> MSLAVLLNKEDKDISDFSKTTAGKSAKKNSRERVADVAPTRVLDKKQAYLSQLNSEFNRIKRRDSIEQLYQDWKFINLQEFELISEWNQQSKDWQFDNTNDSQDLHFKKLYRDMSMINKEWAEYQSFKNANLSDIINEKDADEDEEDDEDELEDGEEDMEEDEASTGRHTNGKSMRGNGIQKSRKKDAAAAAAIGKAIKDDQTHADTVVTVNGDENEDGNNGEDEDNDNDNENNNDNDNDNENENDNDSDNDDEEENGEEDEEEEEIEDLDEEDFAAFEEQDDNDDEDFNPDVEKRRKRSSSSSSSTKLSMNSLSLITSKKINKNITINSDRPKIVRELIKMCNKNKHQKIKKRRFTNCIVTDYNPIDSKLNIKITLKQYHVKRLKKLINDAKREREREEALKNNVGLDGNDLDNDEDGSESHKRRKLNNNTANGADDANKRKFNTRHGLPTYGMKMNAKEARAIQRHYDNTYTTIWKDMARKDSTKMSRLVQQIQSIRSTNFRKTSSLCAREAKKWQSKNFKQIKDFQTRARRGIREMSNFWKKNEREERDLKKKIEKEAMEQAKKEEEEKESKRQAKKLNFLLTQTELYSHFIGRKIKTNELEGNNVSSNDSESQKNIDISALAPNKNDFHAIDFDNENDEQLRLRAAENASNALAETRAKAKQFDDHANAHEEEEEEDELNFQNPTSLGEITIEQPKILACTLKEYQLKGLNWLANLYDQGINGILADEMGLGKTVQSISVLAHLAENHNIWGPFLVVTPASTLHNWVNEISKFLPQFKILPYWGNANDRKVLRKFWDRKNLRYNKNAPFHVMVTSYQMVVTDANYLQKMKWQYMILDEAQAIKSSQSSRWKNLLSFHCRNRLLLTGTPIQNSMQELWALLHFIMPSLFDSHDEFNEWFSKDIESHAEANTKLNQQQLRRLHMILKPFMLRRVKKNVQSELGDKIEIDVLCDLTQRQAKLYQVLKSQISTNYDAIENAATNDSTSNSASNSGSDQNLINAVMQFRKVCNHPDLFERADVDSPFSFTTFGKTTSMLTASVANNNSSVISNSNMNLSSMSSNNISNGKFTDLIYSSRNPIKYSLPRLIYEDLILPNYNNDVDIANKLKNVKFNIFNPSTNYELCLFLSKLTGEPSLNEFFRVSTTPLLKRVIERTNGPKNTDSLSFKTITQELLEVTRNAPSEGVMASLLNVEKHAYEREYLNCIQRGYHPNVSAPPVTIEVLGSSHVTNSINNELFDPLISQALSDIPAITQYNMHVKKGIPVEDFPKTGLFPEPLNKNFSSNISMPSMDRFITESAKLRKLDELLVKLKSEGHRVLIYFQMTKMMDLMEEYLTYRQYNHIRLDGSSKLEDRRDLVHDWQTNPEIFVFLLSTRAGGLGINLTAADTVIFYDSDWNPTIDSQAMDRAHRLGQTRQVTVYRLLVRGTIEERMRDRAKQKEQVQQVVMEGKTQEKNIKTIEVGENDSEVTREGSKSISQDGIKEAASALA;> MSSRDASLTPLKAVVIDDPPLRQTPEPFDEQSAYNPQSPIAIDFGSSKLRAGFVNHATPTHIFPNALTKFRDRKLNKNFTFVGNDTLLDQAVRSQSRSPFDGPFVTNWNLTEEILDYTFHHLGVVPDNGIPNPILLTERLATVQSQRTNWYQILFETYNVPGVTFGIDSLFSFYNYNPSGNKTGLVISCGHEDTNVIPVVDGAGILTDAKRINWGGHQAVDYLNDLMALKYPYFPTKMSYLQYETMYKDYCYVSRNYDEDIEKILTLENLDTNDVVVEAPFTEVLQPQKTEEELRIQAEKRKETGKRLQEQARLKRMEKLVQKQEEFEYFSKVRDQLIDEPKKKVLSVLQNAGFDDERDFKKYLHSLEQSLKKAQMVEAEDDSHLDEMNEDKTAQKFDLLDIADEDLNEDQIKEKRKQRFLKASQDARQKAKEEKERVAKEEEEKKLKEQQWRETDLNGWIKDKRLKLNKLIKRRKEKLKLRDEMKDRKSQVSQNRMKNLASLAEDNVKQGAKRNRHQATIDNDPNDTFGANDEDWLIYTDITQNPEAFEEALEYEYKDIVELERLLLEHDPNFTEEDTLEAQYDWRNSILHLFLRGPRPHDSENIHEQHQMHLNVERIRVPEVIFQPTMGGQDQAGICELSETILLKKFGSQPGKLSQTSIDMVNNVLITGGNAKVPGLKERIVKEFTGFLPTGTNITVNMSSDPSLDAWKGMAALARNEEQYRKTVISKKEYEEYGPEYIKEHKLGNTKYFED;> MSGSRGNSSNSSVSNNSNNNNNNDGGDERLLFLRSVGERNEIGFPSRFKSAHYKKPTRRHKSARQLISDENKRINALLTKANKAAESSTAARRLVPKATYFSVEAPPSIRPAKKYCDVTGLKGFYKSPTNNIRYHNAEIYQLIVKPMAPGVDQEYLKLRGANFVLK;>MVAISEVKENPGVNSSNSGAVTRTAAHTHIKGLGLDESGVAKRVEGGFVGQIEAREACGVIVDLIKAKKMSGRAILLAGGPSTGKTALALAISQELGPKVPFCPLVGSELYSVEVKKTETLMENFRRAIGLRIKETKEVYEGEVTELTPEDAENPLGGYGKTISHVIVGLKSAKGTKTLRLDPTIYESIQREKVSIGDVIYIEANTGAVKRVGRSDAYATEFDLETEEYVPLPKGEVHKKKEIVQDVTLHDLDVANARPQGGQDVISMMGQLLKPKKTEITEKLRQEVNKVVAKYIDQGVAELIPGVLFIDEVNMLDIEIFTYLNKALESNIAPVVVLASNRGMTTVRGTEDVISPHGVPPDLIDRLLIVRTLPYDKDEIRTIIERRATVERLQVESSALDLLATMGTETSLRYALQLLAPCGILAQTSNRKEIVVNDVNEAKLLFLDAKRSTKILETSANYL[3x];>MSIQTSDPNETSDLKSLSLIAAHSHITGLGLDENLQPRPTSEGMVGQLQARRAAGVILKMVQNGTIAGRAVLVAGPPSTGKTALAMGVSQSLGKDVPFTAIAGSEIFSLELSKTEALTQAFRKSIGIKIKEETELIEGEVVEIQIDRSITGGHKQGKLTIKTTDMETIYELGNKMIDGLTKEKVLAGDVISIDKASGKITKLGRSFARSRDYDAMGADTRFVQCPEGELQKRKTVVHTVSLHEIDVINSRTQGFLALFTGDTGEIRSEVRDQINTKVAEWKEEGKAEIVPGVLFIDEVHMLDIECFSFINRALEDEFAPIVMMATNRGVSKTRGTNYKSPHGLPLDLLDRSIIITTKSYNEQEIKTILSIRAQEEEVELSSDALDLLTKTGVETSLRYSSNLISVAQQIAMKRKNNTVEVEDVKRAYLLFLDSARSVKYVQENESQYIDDQGNVQISIAK[3x];> MDSEASDIEAELSDSVSAGGEEYIDDDDYTEDIDDQIVTAKSSRRTARRSVPKGVRTSKRIRDKELSVEVDEDYDEEEDVLSPSKKRHLHTRSMDKRQVAATASEKSDIGDSKGNDGEIEDGILEEEESLEKELNRGGGKEVEKSEESYYAQNDVGQKGEEEQDGESGGYEDNEPSISKESDELVSVVNGNGNEEDDEVEATKENTTDSTRSTTTRSKMLLDLLEDGGSKKKLTDEEIQLRRAENARKRKNLSEKRLEEEKQDTINKLLKKRAGKSRSHLPNDDEKNDGSSSFVKPRRPYNSEGMTRILRRYEEDLFCTF

However, amongst these remodelers, the INO80 chromatin remodeler appears largely sufficient to generate the well positioned +1 and −1 nucleosomes. S.c INO80 is a multi-subunit complex consisting of 15 subunits that are divided into three different modules. The catalytic module with the Ino80 (ATPase) RecA lobes and insert, Arp5, Ies6, Ies2, Rvb1 and Rvb2, constitutes the core unit of INO80 (C-module). INO80 slides nucleosomes with 40 bp of flanking DNA ~100-fold slower than nucleosomes with 80 bp of flanking DNA, displaying a switch like response to flanking DNA length.

INO80 complexes lacking the Arp8 module (ΔArp8) were purified from yeast strains lacking the Arp8 subunit, which results in the absence of the entire module. To test this possibility structurally, we determined the cryo-EM structure of ΔArp8 INO80 bound to S.c 0/40 nucleosomes in the presence of ADP/BeFx. The overall architecture of the C-module of ΔArp8 INO80 bound to 0/40 nucleosomes is again similar to that observed with WT INO80 bound to S.c 0/40 and 0/80. However, the density corresponding to the HSA around the Ino80 motor domain that was observed with the Arp8 module in WT INO80 is no longer detectable. This is likely because, without the Arp8 module, the HSA region is either poorly structured or highly dynamic. We interpret the absence of HSA density as indicative of an activated state, where the HSA is no longer held in an inactive conformation by the Arp8 module. Deletion of the Arp8 module resulted in only a moderate decrease (~2-fold) in sliding of S.c 0/80 nucleosomes. In contrast, this deletion resulted in a ~75-fold increase in remodeling of S.c 0/40 nucleosomes. As a result, in the absence of the Arp8 module, INO80 remodeled both 0/40 and 0/80 nucleosomes rapidly and with comparable kinetics, and the sliding activity of INO80 was not dependent on flanking DNA length.> MADYKDDDDKSGPDEVDASGRMACWPQLRLLLWKNLTFRRRQTCQLLLEVAWPLFIFLILISVRLSYPPYEQHECHFPNKAMPSAGTLPWVQGIICNANNPCFRYPTPGEAPGVVGNFNKSIVARLFSDARRLLLYSQKDTSMKDMRKVLRTLQQIKKSSSNLKLQDFLVDNETFSGFLYHNLSLPKSTVDKMLRADVILHKVFLQGYQLHLTSLCNGSKSEEMIQLGDQEVSELCGLPREKLAAAERVLRSNMDILKPILRTLNSTSPFPSKELAEATKTLLHSLGTLAQELFSMRSWSDMRQEVMFLTNVNSSSSSTQIYQAVSRIVCGHPEGGGLKIKSLNWYEDNNYKALFGGNGTEEDAETFYDNSTTPYCNDLMKNLESSPLSRIIWKALKPLLVGKILYTPDTPATRQVMAEVNKTFQELAVFHDLEGMWEELSPKIWTFMENSQEMDLVRMLLDSRDNDHFWEQQLDGLDWTAQDIVAFLAKHPEDVQSSNGSVYTWREAFNETNQAIRTISRFMECVNLNKLEPIATEVWLINKSMELLDERKFWAGIVFTGITPGSIELPHHVKYKIRMDIDNVERTNKIKDGYWDPGPRADPFEDMRYVWGGFAYLQDVVEQAIIRVLTGTEKKTGVYMQQMPYPCYVDDIFLRVMSRSMPLFMTLAWIYSVAVIIKGIVYEKEARLKETMRIMGLDNSILWFSWFISSLIPLLVSAGLLVVILKLGNLLPYSDPSVVFVFLSVFAVVTILQCFLISTLFSRANLAAACGGIIYFTLYLPYVLCVAWQDYVGFTLKIFASLLSPVAFGFGCEYFALFEEQGIGVQWDNLFESPVEEDGFNLTTSVSMMLFDTFLYGVMTWYIEAVFPGQYGIPRPWYFPCTKSYWFGEESDEKSHPGSNQKRISEICMEEEPTHLKLGVSIQNLVKVYRDGMKVAVDGLALNFYEGQITSFLGHNGAGKTTTMSILTGLFPPTSGTAYILGKDIRSEMSTIRQNLGVCPQHNVLFDMLTVEEHIWFYARLKGLSEKHVKAEMEQMALDVGLPSSKLKSKTSQLSGGMQRKLSVALAFVGGSKVVILDEPTAGVDPYSRRGIWELLLKYRQGRTIILSTHHMDEADVLGDRIAIISHGKLCCVGSSLFLKNQLGTGYYLTLVKKDVESSLSSCRNSSSTVSYLKKEDSVSQSSSDAGLGSDHESDTLTIDVSAISNLIRKHVSEARLVEDIGHELTYVLPYEAAKEGAFVELFHEIDDRLSDLGISSYGISETTLEEIFLKVAEESGVDAETSDGTLPARRNRRAFGDKQSCLRPFTEDDAADPNDSDIDPESRETDLLSGMDGKGSYQVKGWKLTQQQFVALLWKRLLIARRSRKGFFAQIVLPAVFVCIALVFSLIVPPFGKYPSLELQPWMYNEQYTFVSNDAPEDTGTLELLNALTKDPGFGTRCMEGNPIPDTPCQAGEEEWTTAPVPQTIMDLFQNGNWTMQNPSPACQCSSDKIKKMLPVCPPGAGGLPPPQRKQNTADILQDLTGRNISDYLVKTYVQIIAKSLKNKIWVNEFRYGGFSLGVSNTQALPPSQEVNDAIKQMKKHLKLAKDSSADRFLNSLGRFMTGLDTKNNVKVWFNNKGWHAISSFLNVINNAILRANLQKGENPSHYGITAFNHPLNLTKQQLSEVALMTTSVDVLVSICVIFAMSFVPASFVVFLIQERV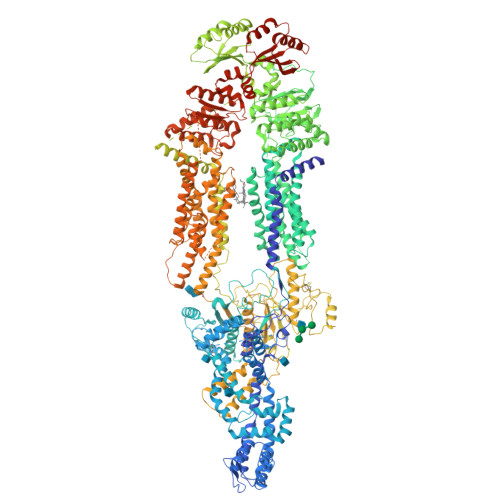SKAKHLQFISGVKPVIYWLSNFVWDMCNYVVPATLVIIIFICFQQKSYVSSTNLPVLALLLLLYGWSITPLMYPASFVFKIPSTAYVVLTSVNLFIGINGSVATFVLELFTDNKLNNINDILKSVFLIFPHFCLGRGLIDMVKNQAMADALERFGENRFVSPLSWDLVGRNLFAMAVEGVVFFLITVLIQYRFFIRPRPVNAKLSPLNDEDEDVRRERQRILDGGGQNDILEIKELTKIYRRKRKPAVDRICVGIPPGECFGLLGVNGAGKSSTFKMLTGDTTVTRGDAFLNKNSILSNIHEVHQNMGYCPQFDAITELLTGREHVEFFALLRGVPEKEVGKVGEWAIRKLGLVKYGEKYAGNYSGGNKRKLSTAMALIGGPPVVFLDEPTTGMDPKARRFLWNCALSVVKEGRSVVLTSHSMEECEALCTRMAIMVNGRFRCLGSVQHLKNRFGDGYTIVVRIAGSNPDLKPVQDFFGLAFPGSVLKEKHRNMLQYQLPSSLSSLARIFSILSQSKKRLHIEDYSVSQTTLDQVFVNFAKDQSDDDHLKDLSLHKNQTVVDVAVLTSFLQDEKVKESYVLEGSDEVDAVEGSHHHHHHHHHH>GAMDIAAQAKLVYHLNKYYNEKCQARKAAIAKTIREVCKVVSDVLKEVEVQEPRFISSLNEMDNRYEGLEVISPTEFEVVLYLNQMGVFNFVDDGSLPGCAVLKLSDGRKRSMSLWVEFITASGYLSARKIRSRFQTLVAQAVDKCSYRDVVKMVADTSEVKLRIRDRYVVQITPAFKCTGIWPRSAAHWPLPHIPWPGPNRVAEVKAEGFNLLSKECHSLAGKQSSAESDAWVLQFAEAENRLQMGGCRKKCLSILKTLRDRHLELPGQPLNNYHMKTLVSYECEKHPRESDWDESCLGDRLNGILLQLISCLQCRRCPHYFLPNLDLFQGK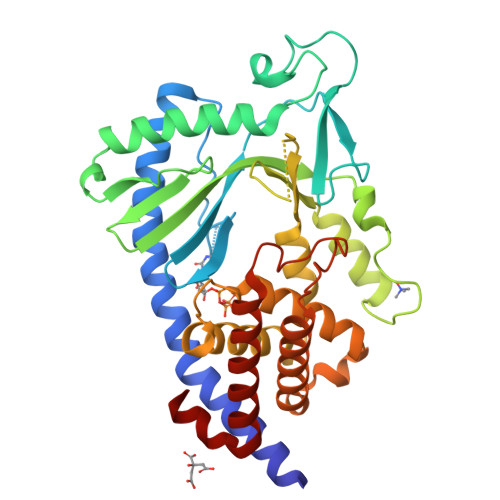PHSALENAAKQTWRLAREILTNPKSLEKL[10x]>[2x]GSMQNRQVANATKVAVAGASGYAGGEILRLLLGHPAYADGRLRIGALTAATSAGSTLGEHHPHLTPLAHRVVEPTEAAVLGGHDAVFLALPHGHSAVLAQQLSPETLIIDCGADFRLTDAAVWERFYGSSHAGSWPYGLPELPGARDQLRGTRRIAVPGCYPTAALLALFPALAADLIEPAVTVVAVSGTSGAGRAATTDLLGAEVIGSARAYNIAGVHRHTPEIAQGLRAVTDRDVSVSFTPVLIPASRGILATCTARTRSPLSQLRAAYEKAYHAEPFIYLMPEGQLPRTGAVIGSNAAHIAVAVDEDAQTFVAIAAIDNLVKGTAGAAVQSMNLALGWPETDGLSVVGVAP

The L-arginine biosynthesis pathway consists of eight enzymes that catalyse the conversion of L-glutamate to L-arginine, appears to be attractive target for anti-Tuberculosis (TB) drug discovery. The arginine biosynthesis pathway consists of eight different enzymes ([Fig fig1]) all considered to be essential for *M. tuberculosis* growth *in vitro*. In this work, the ligandability of four enzymes of the pathway ArgB, ArgC, ArgD and ArgF is explored using a fragment-based approach. In conclusion, using a fragment-based approach, we have discovered inhibitors that bind to novel sites in ArgB and ArgF and to the active sites of ArgC and ArgD, which in case of ArgB show on target activity against *M. tuberculosis*.

Additionally, structures were solved with 4 fragment binders, occupying either of the two distinct pockets: the substrate-binding ([Fig fig2] and [Fig fig2]) and the NADP(H)-binding pockets ([Fig fig2] and [Fig fig2]). As compared to NMR571, NMR322 binds deeper in the pocket ([Fig fig2] and [Fig fig2]). Enzymatic assays revealed that 2 mM NMR322 inhibited ArgC activity by 45% whereas 2 mM NMR571 caused a 37% inhibition. Although the thermal shifts obtained for NADP(H)-binding pocket fragments NMR401 and NMR863 were higher than those for substrate-binding pocket fragments NMR322 and NMR571, the SPR binding response for the latter was better and positively correlated with percentage inhibition of enzymatic activity (**[Table tbl2]**). Our results further show that in the case of ArgC there are two possible strategies to develop inhibitors, with one targeting the cofactor binding site and the other the substrate binding site. It is not clear at this point which strategy has the highest potential to result in potent inhibitors.> V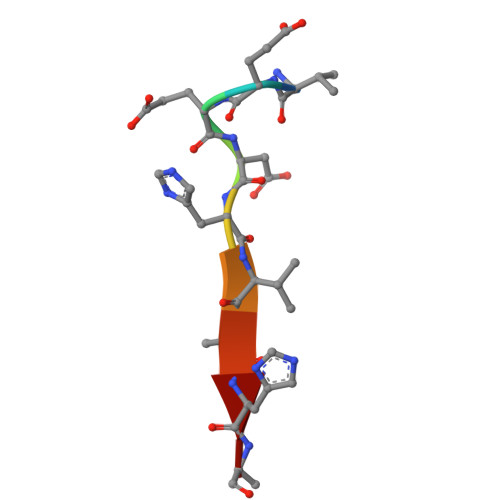EEDHVAHA> IKGGLFADIASHPWQAAIFAKHRRSPGERFLCGGILISSCWILSAAHCFQERFPPHHLTVILGRTYRVVPGEEEQKFEVEKYIVHKEFDDDTYDND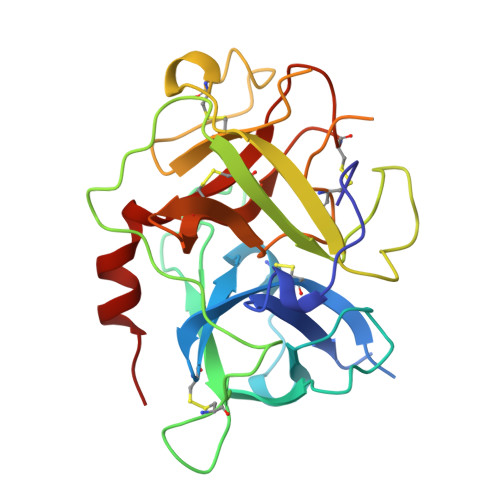IALLQLKSDSSRCAQESSVVRTVCLPPADLQLPDWTECELSGYGKHEALSPFYSERLKEAHVRLYPSSRCTSQHLLNRTVTDNMLCAGDTRSGGPQANLHDACQGDSGGPLVCLNDGRMTLVGIISWGLGCGQKDVPGVYTKVTNYLDWIRDNMRP>GMTTTQPEAKDRISSLPVPDATQVPEGVRKLWAKAEANIGFVPNVFRAQAVNGEQFLAWWNYFNLLLNKEGYLTNAERELVAVVVSGVNRCLYCAVSHGAALREFLGDPQKADAVAVNWRHADLTEREQALAAYAEKLTRHPAE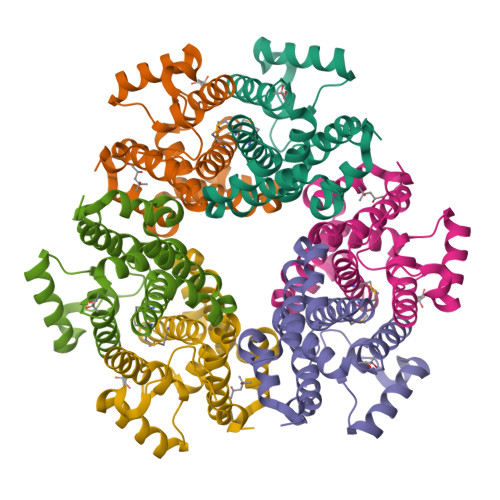VTAADLEPLRAVGLDDHQIMELVQVIGMFNLTNRVSSALGFVPNPEYYRQAR[2x]> ADEPVWRSEQAIGAIAASQEDGVFVASGSCLDQLDYSLEHSLSRLYRDQAGNCTEPVSLAPPARPRPGSSFSKLLLPYREGAAGLGGLLLTGWTFDRGACEVRPLGNLSRNSLRNGTEVVSCHPQGSTAGVVYRAGRNNRWYLAVAATYVLPEPETASRCNPAASDHDTAIALKDTEGRSLATQELGRLKLCEGAGSLHFVDAFLWNGSIYFPYYPYNYTSGAATGWPSMARIAQSTEVLFQGQASLDCGHGHPDGRRLLLSSSLVEALDVWAGVFSAAAGEGQERRSPTTTALCLFRMSEIQARAKRVSWDFKTAESHCKEGDQPERVQPIASSTLIHSDLTSVYGTVVMNRTVLFLGTGDGQLLKVILGENLTSNCPEVIYEIKEETPVFYKLVPDPVKNIYIYLTAGKEVRRIRVANCNKHKSCSECLTATD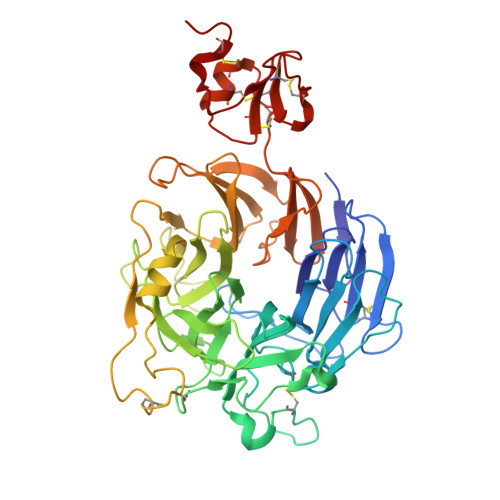PHCGWCHSLQRCTFQGDCVHSENLENWLDISSGAKKCPGAP>MNRDDAFLTVQARLGYDFSGDMKIGGKYTSLIEHAGLAYMSGQIPRVEDKVQVCGKVGF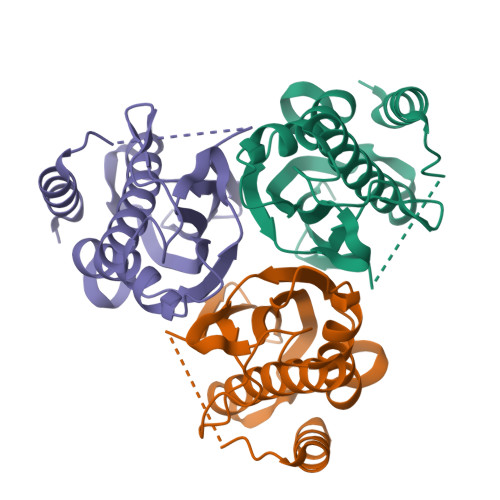DVDLSQAQLAASISTMRALAILKQHYGTLQVVEKVLQMNVFIHSTADFTQQSEVADGASEILYEILGSDTGQHTRTSVSVCQLPKNASVEINFIVALKQNNGQE[9x]> AGPTAVPLGTAGNYAILASAGVSTVPQSVITGAVGLSPAAATFLTGFSLTMSSTGTFSTSTQVTGQLTAADYGTPTPSILTTAIGDMGTAYVNAATRSGPNFLEIYTGALGGKILPP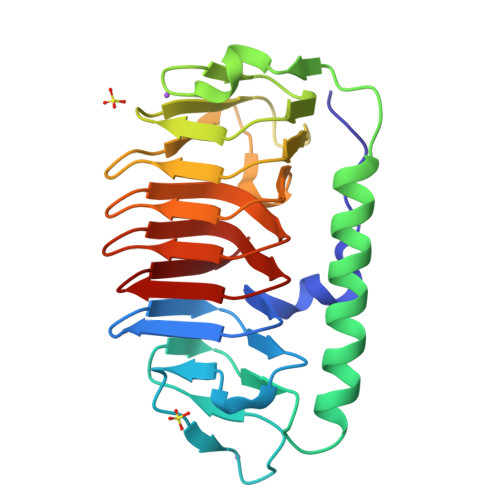GLYKWTSPVGASADFTIIGTSTDTWIFQIAGTLGLAAGKKIILAGGAQAKNIVWVVAGAVSIEAGAKFEGVILAKTAVTLKTGSSLNGRILSQTAVALQKATVVQK> MKKVVAVVKLQLPAGKATPAPPVGPALGQHGANIMEFVKAFNAATANMGDAIVPVEITIYADRSFTFVTKTPPASYLIRKAAGLEKGAHKPGREKVGRITWEQVLEIAK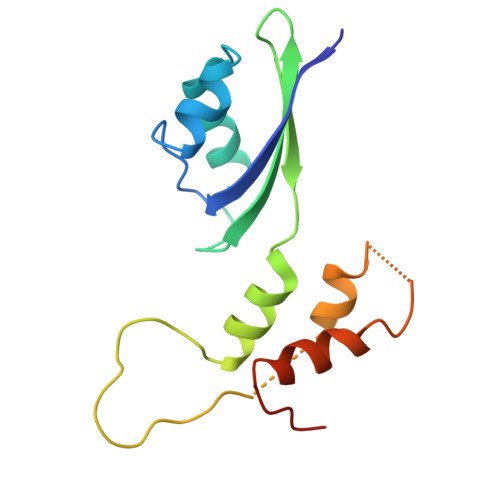QKMPDLNTTDLEAAARMIAGSARSMGVEVVGAPEVKDA> PPGTVDKKMVEKCWKLMDKVVRLCQNPKLALKNSPPYILDLLPDTYQHLRTILSRYEGKMETLGENEYFRVFMENLMKKTKQTISLFKEGKERMYEENSQPRRNLTKLSLIFSHMLAELKGIFPSGLFQGDTFRITKADAAEFWRKAFGEKTIVPWKS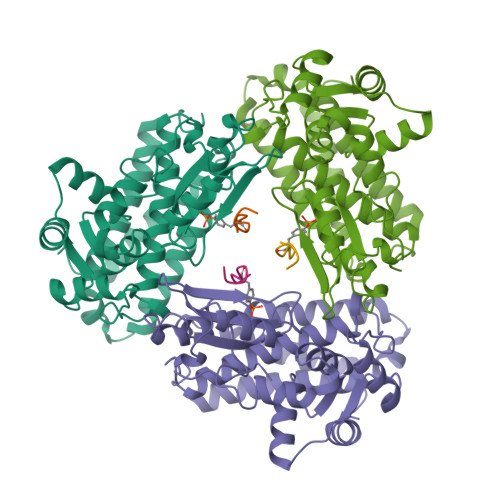FRQALHEVHPISSGLEAMALKSTIDLTCNDYISVFEFDIFTRLFQPWSSLLRNWNSLAVTHPGYMAFLTYDEVKARLQKFIHKPGSYIFRLSCTRLGQWAIGYVTADGNILQTIPHNKPLFQALIDGFREGFYLFPDGRNQNPDLTG;> TLNSDGYTPEPA> TLTEDLDAPQDTGNIENGAADNSPQPRTTFDYTGNPLPPDTKLENFFSFYRLLPMGGSGAPSLSFPADEGTIIPLNPINWLKGADVSGIAAMLSCFTYIAADLRITLRFSNPNDNPATMLVAFAPPGATIPLKPTRQMLSNFYMAEVPVSAATSTMVSFSIPYTSPLSAIPTSYFGWEDWSGTNFGQLSSGSWGNLMLIPSLSVDSAIPFDFQLSCWVAFGNFKAWVPRPPPPLPPLPTPAANAERTVAVIKQ;> GNSVTNIYGNGNNVTTDVGANGWAPTVSTGLGDGPVSASADSLPGRSGGASSEKTHTVSGSSNKVGSRFSKWWEPAAARASESATDSAIEGIDAAGKAASKAITRKLDRPAAPSSTANPQPSLIALNPSATQSGNASILTGSTAPSLLAYPTATPVPLPNPDEPSQPGPSGDRTWLLDTVTWSQEFTRGWNIAGSNGMQWTGLESLIFPVSTDTNWTSTSSPTAYPLPFSFVRAYPDSSWAAMYNTHSMWNCGWRVQVTVNGSQFHAGALILYMVPEATTHAIQTARDNAGFVFPYVILNLYESNTATIEVPYISPTPNTSSGLHAPWTFYLQVLSPLNPPPSLPTSLSCSIYVTPVDSSFHGLRYLAPQ;> HWKTRAVPGAGTFGSAVAGQELPLCGVRAYYPPNAYIPAQVRDWLEFAHRPGLMATVPWTMADEPAERLGIFPVSPSAIAGTGAPISYVISLFSQWRGELAAHLLFTGSAQHYGRLVVCYTPAAPQPPSTMQEAMRGTYTVWDVNAASTLEFTIPFISNSYWKTVDVNNPDALLSTTGYVSIWVQNPLVGPHTAPASALVQAFISAGESFNVRLMQNPALTSQ

Aichi virus 1 (AiV1) is a member of the Kobuvirus genus belonging to the Picornaviridae family of small non-enveloped viruses. The capsid of AiV1 is composed of 60 copies of each of the three capsid proteins VP0, VP1 and VP3 organized with icosahedral symmetry. The outer diameter of the virion is about 300 Å. The AiV1 genome is a single-stranded positive-sense RNA 8251 nucleotides in length.

Here, we report the structure determination of an AiV1 virion based on diffraction data affected by perfect hemihedral twinning. The AiV1 crystal diffracted to a resolution of 2.1 Å. The unit-cell volume and the rotation-function plots indicated that a crystal with the same unit-cell parameters but with I23 symmetry (a subset of I432 symmetry) would allow the packing of AiV1 virions. This provided evidence that the crystal may be hemihedrally twinned, with the two domains composed of I23 unit cells rotated 90° relative to each other. Superimposition of the icosahedral symmetry with the cubic 23 symmetry resulted in the crystallographic asymmetric unit containing five icosa­hedral asymmetric units (1/12 of a virus particle). Based on the orientation of the icosahedral particle and the crystal-packing considerations, the virus particle had to be positioned with its centre at the origin of the unit cell. The procedure permitted the structure to be determined from a molecular-replacement model that had 16% sequence identity and a 1.6 Å r.m.s.d. for Cα atoms in comparison to the crystallized structure. The NCS averaging procedure reduced the model bias introduced by the differences between the molecular-replacement model and the crystallized structure. The electron-density map obtained after 30 cycles of real-space NCS averaging combined with detwinning was interpretable for most of the AiV1 structure. However, some regions, including the surface loops of VP1 located close to the icosahedral fivefold axes and the N-terminal arms of the capsid proteins located on the inside of the capsid, were difficult to interpret. The final AiV1 model includes residues 1–83 and 88–233 of VP1, residues 13–55, 64–75 and 112–370 of VP2 and residues 1–220 of VP3 together with 173 water molecules within one icosahedral asymmetric unit of the virion.> GSMTTERVKKLRVVEDKHVNYKVFIYDHIRQIAIPTTNLNSQSSLEDIIDESTSCQSVSTDGSIEIDGLTLIHNFLSESEESKILNMIDTVEWAQSQSGRRKQDYGPKVNFKHKKVKTDTFVGMPEYADMLLNKMSEYDVKKLGNYQPFEMCNLEYEEVKKSAIEM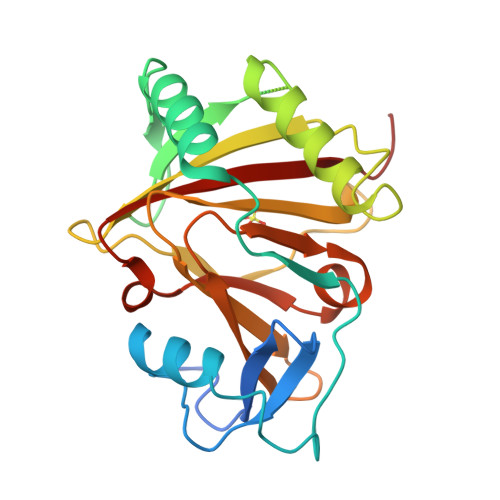HQDDMWIWGNRLISINLINGSVMTLSNDNKSFLCYVHMPHRSLLCMADECRYDWKHGVLAHHIRGRRIALTMREAAKDFA[(2-amino-6-oxo-6,9-dihydro-1H-purin-8-yl)sulfanyl]acetic 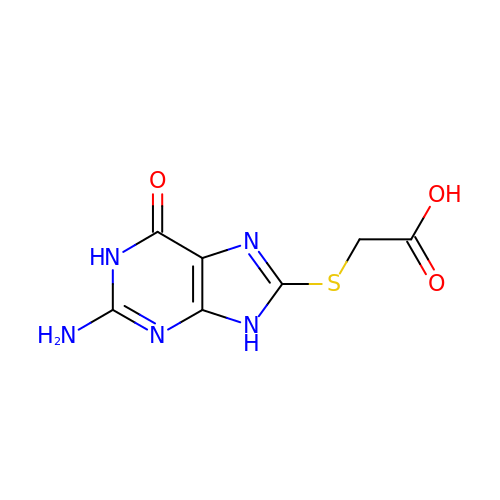acid | C7 H7 N5 O3 S | XIPJLLJJHOEGQG-UHFFFAOYSA-N>[2x]MHTLYAPGGYDIMGYLIQIMNRPNPQVE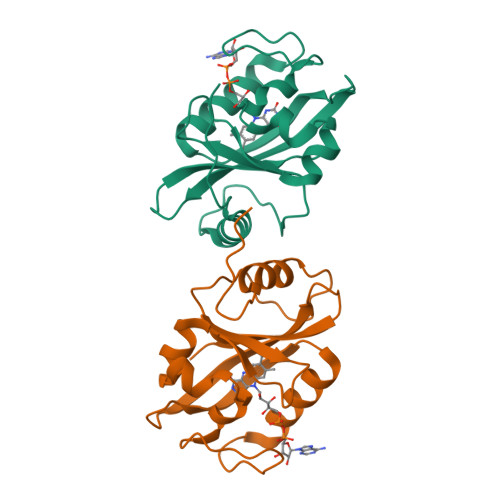LGPVDTSVALILCDLKQKDTPIVYASEAFLYMTGYSNAEVLGRNCRFLQSPDGMVKPKSTRKYVDSNTINTMRKAIDRNAEVQVEVVNFKKNGQRFVNFLTMIPVRDETGEYRYSMGFQCE> MEKKTIVLGVIGSDCHAVGNKILDHAFTNAGFNVVNIGVLSPQELFIKAAIETKADAILVSSLYGQGEIDCKGLRQKCDEAGLEGILLYVGGNIVVGKQHWPDVEKRFKDMGYDRVYAPGTPPEVGIAD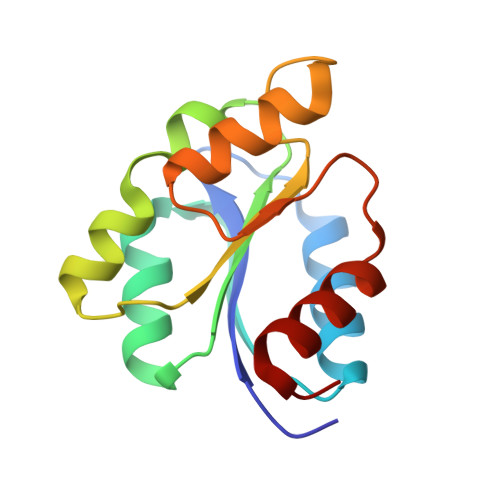LKKDLNIE>GAAGDGAGASRQRKLEALIRDPRSPINVESLLDGLNSLVLDLDFPALRKNKNIDNFLNRYEKIVKKIRGLQMKAEDYDVVKVIGRGAFGEVQLVRHKASQKVYAMKLLSKFEMIKRSDSAFFWEERDIMAFANSPWVVQLFYAFQDDRYLYMVMEYMPGGDLVNLMSNYDVPEKWAKFYTAEVVLALDAIHSMGLIHRDVKPDNMLLDKHGHLKLADFGTCMKMDETGMVHCDTAVGTPDYISPEVLKSQGGDGFYGRECDWWSVGVFLYEMLVGDTPFYADSLVGTYSKIMDH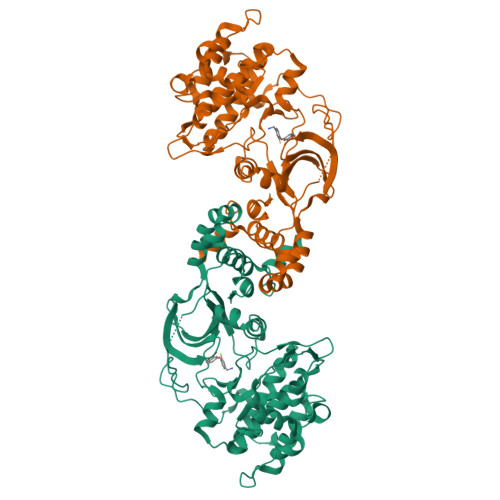KNSLCFPEDAEISKHAKNLICAFLTDREVRLGRNGVEEIRQHPFFKNDQWHWDNIRETAAPVVPELSSDIDSSNFDDIEDDKGDVETFPIPKAFVGNQLPFIGFTYYR[2x]> SELIVNVINGPSLGRLGRREPAVYGGTTHDELVALIEREA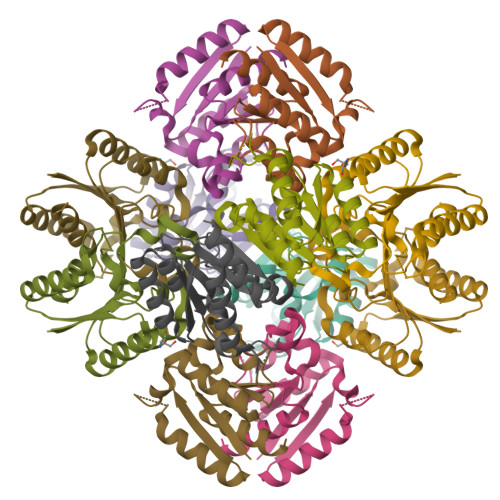AELGLKAVVRQSDSEAQLLDWIHQAADAAEPVILNAGGLTHTSVALRDACAELSAPLIEVHISNVHAREEFRRHSYLSPIATGVIVGLGIQGYLLALRYLAEHVGT>MFYINSKYKIDLDKIMTKMKNKSVINIDDVDDEELLAILYTSKQFEKILKNNEDSKYLENKVFCSVFLEPSTRTRCSFDAAILKLGSKVLNITDMNSTSFYKGETVEDAFKILSTYVDGIIYRDPSKKNVDIAVSSSSKPIINAGNGTGEHPTQSLLDFYTIHNYFPFILDRNINKKLNIAFVGDLKNGRTVHSLSKLLSRYNVSFNFVSCKSLNIPKDIVNTITYNLKKNNFYSDDSIKYFDNLEEGLEDVHIIYMTRIQKERFTDVDEYNQYKNAFILSNKTLENTRDDTKILHPLPRVNEIKVEVDSNPKSVYFTQAENGLYVRMALLYLIFSSTSSAW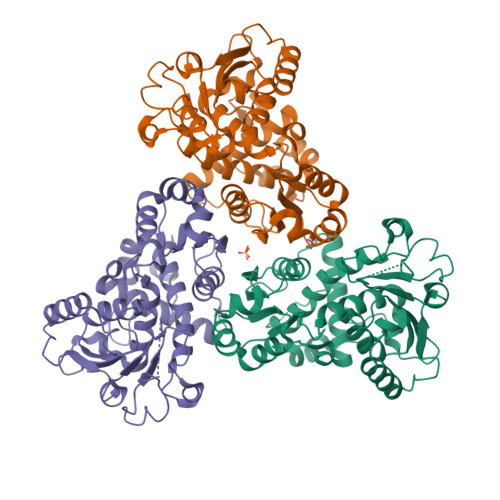SHPQFEK[3x]>QDDASDRQTREVLDPIVASLMEAQQIPGMAIALVRPEGTTISHYGAADRETGTPVDDDTLFEIGSLSKTLTATLASLAEVEGKLDFDAPVSRYLPELEGSAFDDISGLNLGTHTGGGLPLFVPDEVTDRASLMAWYREWQPTEPIGESRTYSNLGIGLLGLETAASLDGEFVPTMRAKVLAPLGMQDTWYDVPEARMADYAMGEDKDGQPTRVSPGVLDDEAYGIKTTAADLAKLVRANLHLADVDAELQQAIDATRQGHYRVGDMTQALIWEQYSLPVAPETLRAGNGYDMILEPNAAEALEPPQSPRDDVWVNKTGSTNGFGGYIVMLPGKHTGLV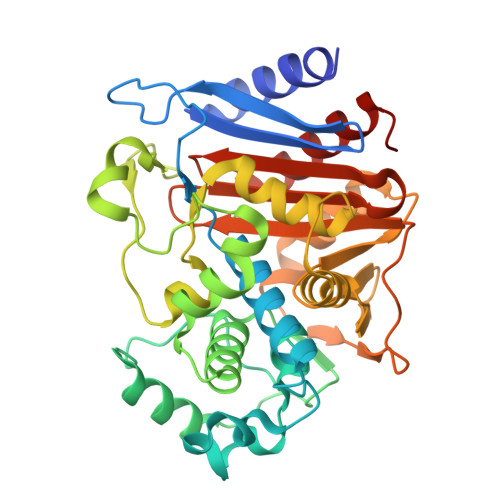MLANKNYPNDARVEAAYRILSGLGAIDVP[3x]>NRVYVHPFNLFSSENISCEVIQSEEHKPLETVHPLPPLPGSTDPDPRTASAAESLKNLTQRTAVLAELQNSLGLRMYQTLSRTQKHTNTLLSPLNAFGALVTLYLGASKKTAISYQQLLGLNLESEQTDCAYFVDGHTVLRTLQAISAHVDESRKELRTLVWTFVNSDADLSKEFLRGTQDFSDDSFVRSVDFSQAKDAEVEVNNFIQKTSDNKVKSMFKGVTPKTDLLFASSVHFKGNWKTAFQPEATSDQDFWTQKNSSVQVPFMMHTGDYKYLDDAGRKCSIVRLGLSKRTFMLLVLPHEGASLQDIEKPLLTVIPTWLRHLKEKYLELSLPKFSLTAVTDLRSVLSEMAVEKYLMGSDASFRRMSSKENFTVDKVLNKVVFEMTEGGSEVQNRTDDGRAPHKVTFNRPFFFAVVEGNSNAILMLGKII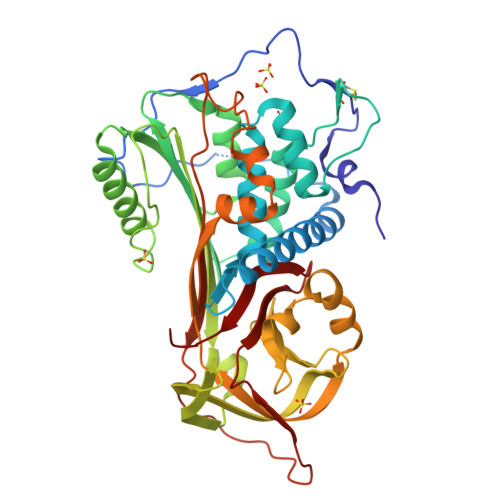NPTA[2x]> GPHMEE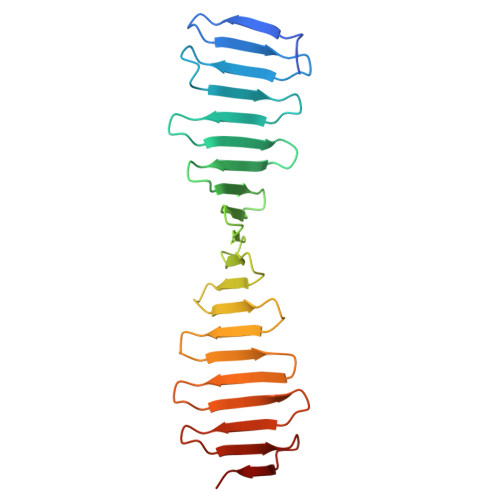IMQSDSKIEKMLPDGGRLVVFPNGTRKELSADGQTVKVMFFNGDVKHTMPDQRVIYYYAEAQTTHITYPDGMEVLQFPNNQTEKHFPDGRKEITFPDQTVKTLHPDGREESVLTDGTIIQLNPDGSKVIQFNTGQREIHTADFKRREYPDGTVKTVYSDGRQETQYPTGRVRLKDPQGKVIMDTKA> DMRPEIRIAQELRRXGDE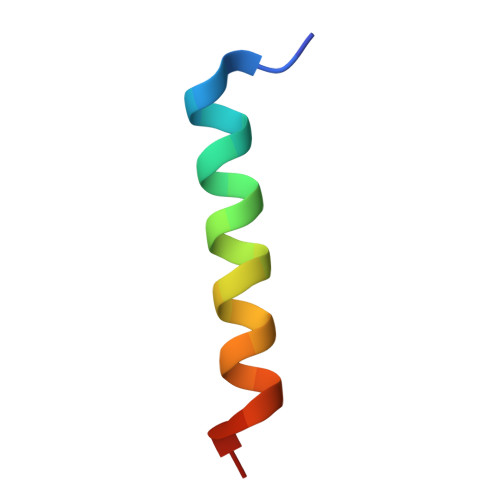FNATYARR>GSMSQAIPSSRVGVKINEWYKMIRQFSVPDAEILKAEVEQDIQQMEEDQDLLIYYSLMCFRHQLMLDYLEPGKTYGNRPTVTELLETIETPQKKLTGLLKYYSLFFRGMYEFDQKEYVEAIGYYREAEKELPFVSDDIEKAEFHFKVAEAYYHMKQTHVSMYHILQALDIYQNHPLYSIRTIQSLFVIAGNYDDFKHYDKALPHLEAALELAMDIQNDRFIAISLLNIANSYDRSGDDQMAVEHFQKAAKVSREKVPDLLPKVLFGLSWTLCKAGQTQKAFQFIEEGLDHITARSHKFYKELFLFLQAVYKETVDERKIHDLLSYFEKKNLHAYIEACARSAAAVFESSCHFEQAAAFYRKVLKAQEDILKGECLYAY[2x];>GSMMNEKILIVDDQYGIRILLNEVFNKEGYQTFQAANGLQALDIVTKERPDLVLLDMKIPGMDGIEILKRMKVIDENIRVIIMTAYGELDMIQESKELGALTHFAKPFDIDEIRDAVKKYLPLKSN[2x]

Rap proteins, named after the founding members of the family, which were shown to be response regulator aspartate phosphatases, have been most thoroughly studied in B. subtilis, where they are central to the regulation of diverse developmental processes including sporulation and genetic competence. A subset of Rap proteins, consisting of RapA, RapB, RapE, and RapH, dephosphorylates Spo0F, consequently reducing the level of phosphorylated Spo0A in the cell and inhibiting sporulation. Signaling converges on the centrally important intermediate response regulator Spo0F, which autophosphorylates using phosphohistidines in a sporulation histidine kinase as a phosphoryl donor. Here we present the RapH-Spo0F X-ray crystal structure, which shows that Rap proteins consist of a 3-helix bundle and a tetratricopeptide repeat domain.

We have determined the X-ray crystal structure of a Rap phosphatase, RapH, in complex with its target protein, Spo0F, which is bound to Mg2+, an important constituent of the Spo0F active site. The single wavelength anomalous diffraction method was used to obtain experimental phases and the RapH-Spo0F structure was ultimately refined to 2.20 Å resolution. The RapH-Spo0F crystallographic asymmetric unit contains RapH-Spo0F complexes in two different conformations, reflecting different steps along the Spo0F dephosphorylation pathway. RapH forms dimers in the RapH-Spo0F crystals; this is consistent with gel filtration studies showing that RapH forms stable dimers in solution. Connected to the C-terminus of the RapH 3-helix bundle via a flexible linker and a short helix (α4) is a large right-handed superhelical domain composed of seven pairs of antiparallel α-helices. The RapH-Spo0F structure revealed that the sidechain of RapH Gln47 inserts into the Spo0F active site. We propose that RapH Gln47 orients water for direct in-line hydrolytic attack on the Spo0F phosphoaspartate-54 phosphorous atom. More specifically, this alignment showed that RapHA binding causes the entire Spo0FA β4-α4 loop to dramatically shift and flip toward the active site. The RapHA-induced conformational change in Spo0FA Thr82 is accompanied by the rotation of the Spo0FA His101 sidechain to an internalized position where it enters space vacated by Thr82. It is important to note that while Spo0F is not phosphorylated in the RapH-Spo0F structure, RapHA locks non-phosphorylated Spo0FA in the conformation corresponding to a phosphorylation-stabilized receiver domain, which is characterized by the rotation of both switch residues and the movement of the β4-α4 loop towards the active site. The entire β4-α4 loop, all of helix α4, and a portion of the α4-β5 loop are disordered in Spo0FB as evidenced by a lack of interpretable electron density corresponding to these residues.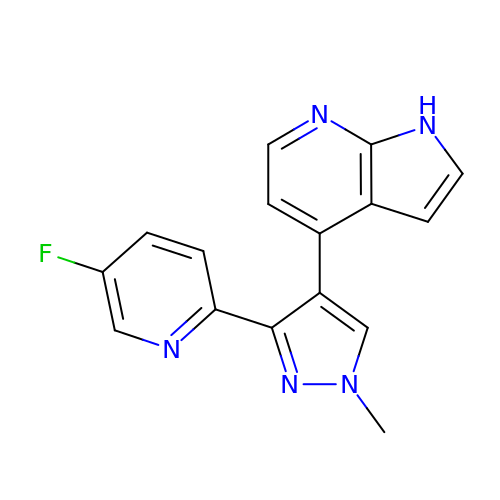(4P)-4-[(3P)-3-(5-fluoropyridin-2-yl)-1-methyl-1H-pyrazol-4-yl]-1H-pyrrolo[2,3-b]pyridine | C16 H12 F N5 | OAUWJBUJGOVSTR-UHFFFAOYSA-N> GHMSHLADVSPPTACRVCGGGVQEFLDLGRQPLSDRFRKPDELDDEFTYRLAVGRCDSCEMVQLTEEVPRDLMFHEVYPYHSSGSSVMREHFAMLARDFLATELTGPDPFIVEIGCNDGIMLRTIQEAGVRHLGFEPSSGVAAKAREKGIRVRTDFFEKATADDVRRTEGPANVIYAANTLCHIPYVQSVLEGVDALLAPDGVFVFEDPYLGDIVAKTSFDQIYDEHFFLFSATSVQGMAQRCGFELVDVQRLPVHGGEVRYTLARQGSRTPSAAVAQLLAAEREQELSDMATLRAFAGNVVKIRDELTALLHRLRAEGRSVVGYGATAKSATVTNFCGIGPDLVHSVYDTTPDKQNRLTPGAHIPVRPASAFSDPYPDYALLFAWNHAEEIMAKEQEFHQA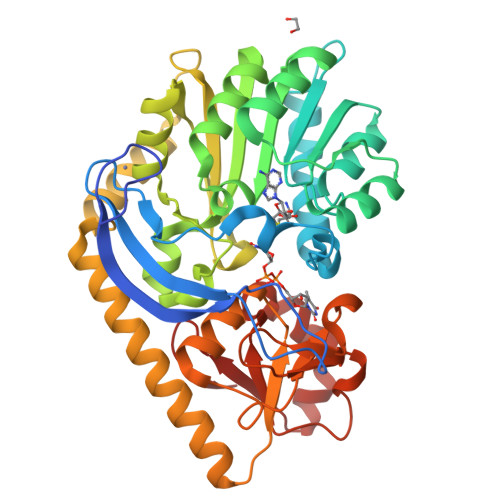GGRWILYVPEVHIR>[2x]MPKRGKKGAVAEDGDELRTEPEAKKSKTAAKKNDKEAAGEGPALYEDPPDQKTSPS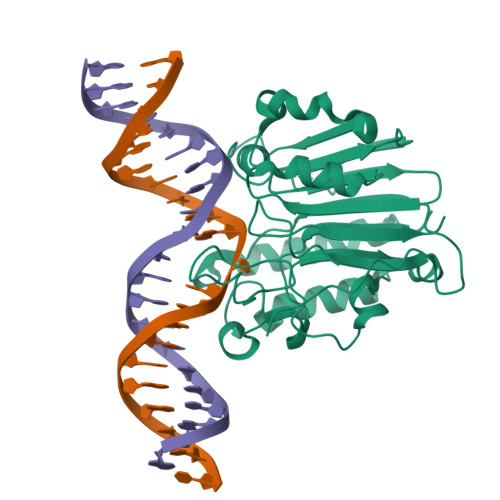GKPATLKICSWNVDGLRAWIKKKGLDWVKEEAPDILCLQQTKCSENKLPAELQELPGLSHQYWSAPSDKEGYSGVGLLSRQAPLKVSYGIGDEEHDQEGRVIVAEFDSFVLVTAYVPNAGRGLVRLEYRQRWDEAFRKFLKGLASRKPLVLCGNLNVAHEEIDLRNPKGNKKNAGFTPQERQGFGELLQAVPLADSFRHLYPNTPYAYTFWTYMMNARSKNVGWRLDYFLLSHSLLPALCDSKIRSKALGSDHCPITLYLAL> MQRSFAALGLWGLSLAQEAHRVAITHPGGSFNQEVAFLFPWVYFFSFLIFLVVAGSLAYVTWKFRARPEDQEEPPQIHGNDRLEVVWTLIPLAIVFVLFGLTAKALIQVNRPIPGAMKVEVTGYQFWWDFHYPELGLRNSNELVLPAGVPVEL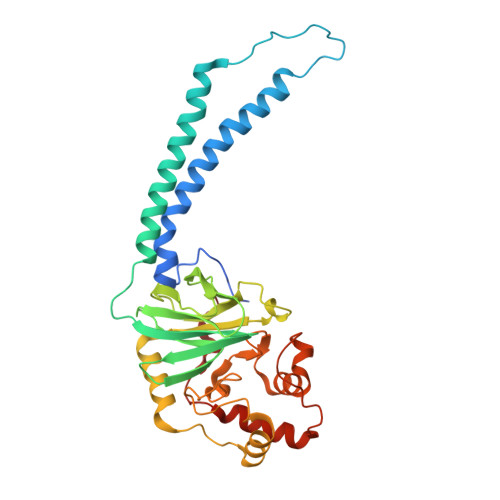EITSKDVIHSFWVPGLAGKRDAIPGQTTRISFEPKEPGLYYGFCAELCGASHARMLFRVVVLPKEEFDRFVEAAKASPAPVADERGQQVFQQNCAACHGVARSMPPAVIGPELGLWGNRTSLGAGIVENTPENLKAWIRDPAGMKPGVKMPGFPQLSEEDLDALVRYLEGLKVEGFDFGALPKF(3beta,5beta,14beta,17alpha)-cholestan-3-ol | C27 H48 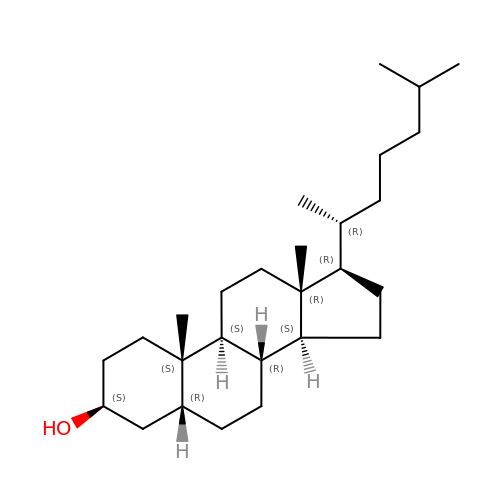O | QYIXCDOBOSTCEI-NWKZBHTNSA-N>MPNIKIFSGSSHQDLSQKIADRLGLELGKVVTKKFSNQETCVEIGESVRGEHVYIVQSGCGEINDNLMELLIMINACKIASASRVTAVIPCFPYARQDKKDKSRAPISAKLVANML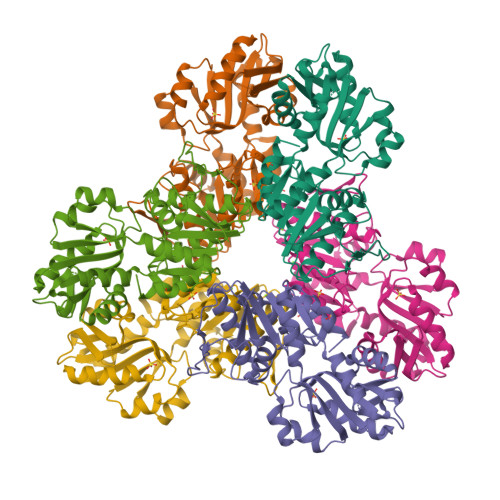SVAGADHIITMDLHASQIQGFFDIPVDNLYAEPAVLKWIRENISEWRNCTIVSPDAGGAKRVTSIADRLNVDFALIHKERKKANEVDRMVLVGDVKDRVAILVDDMADTCGTICHAADKLLSAGATRVYAILTHGIFSGPAISRINNACFEAVVVTNTIPQEDKMKHCSKIQVIDISMILAEAIRRTHNGESVSYLFSHVPLLEHHHHHH[2x]>MAGNKPFNKQQAEPRERDPQVAGLKVPPHSIEAEQSVLGGLMLDNERWDDVAERVVADDFYTRPHRHIFTEMARLQESGSPIDLITLAESLERQGQLDSVGGFAYLAELSKNTPSAANISAYADIVRERAVVREMISVANEIAEAGFDPQGRTSEDLLDLAESRVFKIAESRANKDEGPKNIADVLDATVARIEQLFQQPHDGVTGVNTGYDDLNKKTAGLQPSDLIIVAARPSMGKTTFAMNLVENAAMLQDKPVLIFSLEMPSEQIMMRSLASLSRVDQTKIRTGQLDDEDWARISGTMGILLEKRNIYIDDSSGLTPTEVRSRARRIAREHG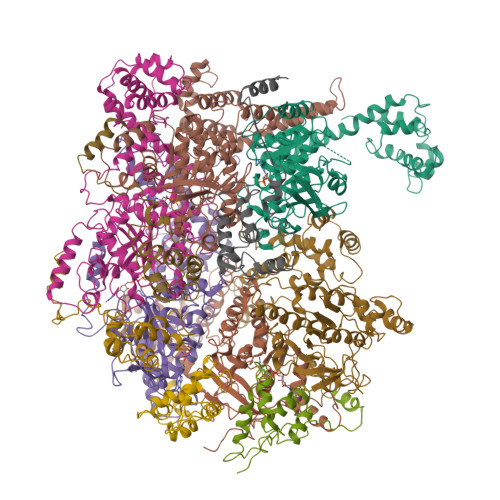GIGLIMIDYLQLMRVPALSDNRTLEIAEISRSLKALAKELNVPVVALSQLNRSLEQRADKRPVNSDLRESGSIEQDADLIMFIYRDEVYHENSDLKGIAEIIIGKQRNGPIGTVRLTFNGQWSRFDNYAGPQYDDE[6x]>[3x]GPDSMTSENPD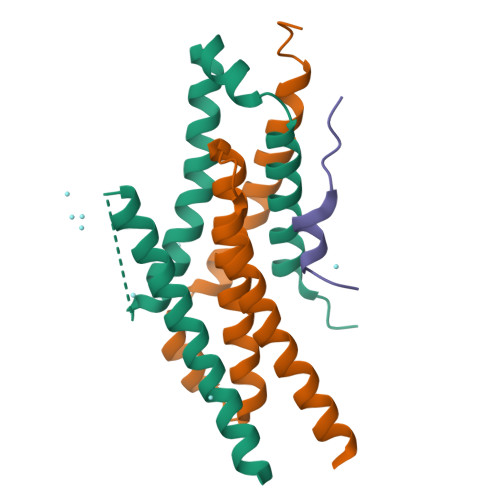VLLSRVINVVRAASSLASQDVDFYKNLDRGFSKDLKSKADKLADMANEIILSIDEHHESFELKEEDISDLWNNFGNIMDNLLEMSDHSLDKLNCAINSKSRGSD;>MEDIEKIKPYVRSFSKALDELKPEIEKLTSKSLDEQLLLLSDERAKLELINRYAYVLSSLMFANMKVLGVKDMSPILGELKRVKSYMDKAKQYDNRITKSNEK[3x];>[3x]MDSTDLFDVFEETPVELPTK> LGSSNDNIELVDFQNIMFYGDAEVGDNQQPFTFILDTGSANLWVPSVKCTTAGCLTKHLYDSSKSRTYEKDGT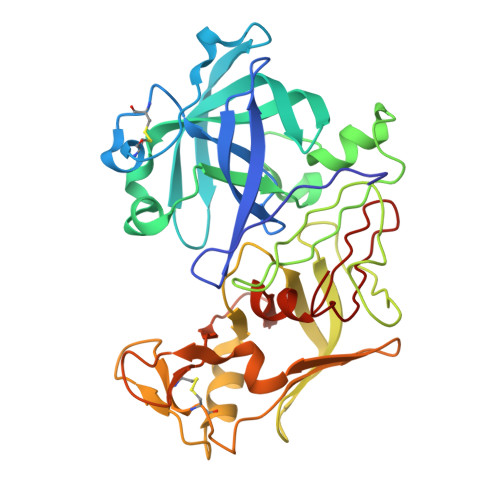KVEMNYVSGTVSGFFSKDLVTVGNLSLPYKFIEVIDTNGFEPTYTASTFDGILGLGWKDLSIGSVDPIVVELKNQNKIENALFTFYLPVHDKHTGFLTIGGIEERFYEGPLTYEKLNHDLYWQITLDAHVGNIMLEKANCIVDSGTSAITVPTDFLNKMLQNLDVIKVPFLPFYVTLCNNSKLPTFEFTSENGKYTLEPEYYLQHIEDVGPGLCMLNIIGLDFPVPTFILGDPFMRKYFTVFDYDNHSVGIALAKKNL> MGSSHHHHHHGSTYDFTGNTPPPAPQGMKWVKISQL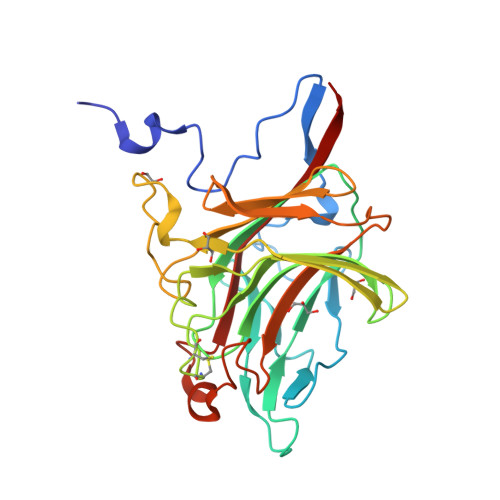SDEFNNGFNTDKWTKSLWNYGVPVQMKAENSGVSDGKLWIKATLGNDPERWFETSRVMSKAQVNYPMYTVSRIKGAHISAYNTFWLNNGNISNRNEIDVIENNSNPSCNCQPDFPWQMNSQYFHVVNDDTKRNKGNFDNRELSDANPLKGVAWNEEYHTFGVWWKDATHIQFYLDGEPAGSVVSARDFTRELNIIWDLWTVDADWLGGLAKKEHLSNNNINTMKIDWIHTYQLVEE7-[[2-[[1-(1-IMINOETHYL)PIPERIDIN-4-YL]OXY]-9H-CARBOZOL-9-YL]METHYL]NAPHTHALENE-2-CARBOXIMIDAMID | C31 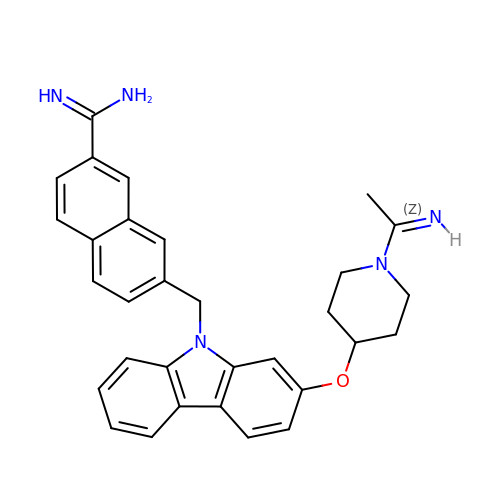H31 N5 O | DZLGSWPXZYDHBD-RGXNXFOYSA-N> MALEEIRPKEVYLDRKLLTLEDKELGSGNFGTVKKGYYQMKKVVKTVAVKILKNEANDPALKDELLAEANVMQQLDNPYIVRMIGICEAESWMLVMEMAELGPLNKYLQQNRHVKDKNIIELVHQVSMGMKYLEESNFVHRDLAARNVLLVTQHYAKISDFGLSKALRADENYYK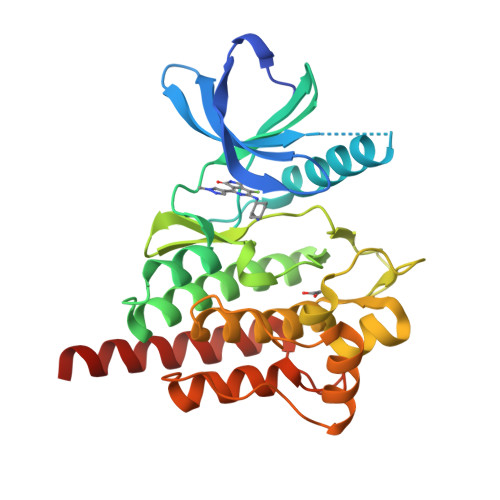AQTHGKWPVKWYAPECINYYKFSSKSDVWSFGVLMWEAFSYGQKPYRGMKGSEVTAMLEKGERMGCPAGCPREMYDLMNLCWTYDVENRPGFAAVELRLRNYYYDVVNHHHHHH> ERHKILHRLL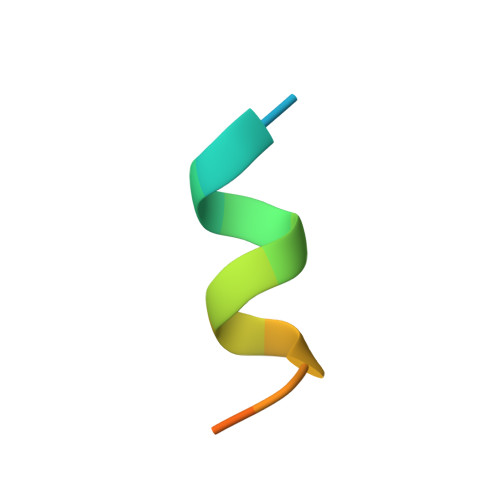QEGSPS> MVLNKWAAVTKSAPPAAGLRPLARTVSPNPKLR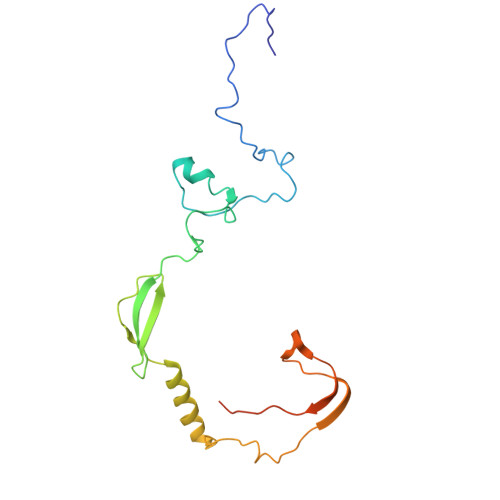PADYKVPYVLRTFIKDRHSSEMQHIENRGMYREELAIERSRFPRMQKTLTIQTDGSLNEREFEFAVPPVVMLFQDRLSAHRQRQVALAKIGKLKRVKSWETSVRGKESLNPVCNALVFPYCVPKKMLVRPRIVDPLSAKSMADNRRSRDDPS>[2x]EEAEET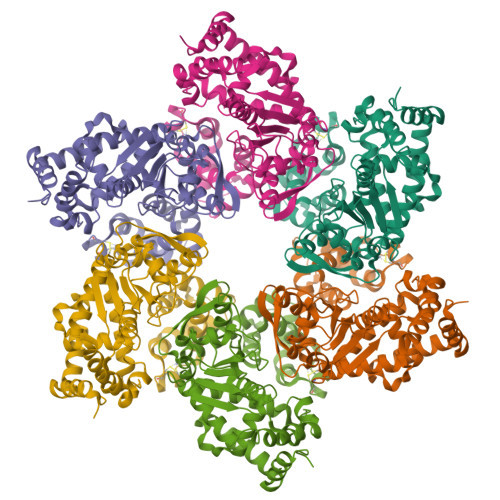KQVSWKLVTEYAMETKCDDVLLLLGMYLEFQYSFEMCLKCIKKEQPSHYKYHEKHYANAAIFADSKNQKTICQQAVDTVLAKKRVDSLQLTREQMLTNRFNDLLDRMDIMFGSTGSADIEEWMAGVAWLHCLLPKMDSVVYDFLKCMVYNIPKKRYWLFKGPIDSGKTTLAAALLELCGGKALNVNLPLDRLNFELGVAIDQFLVVFEDVKGTGGESRDLPSGQGINNLDNLRDYLDGSVKVNLEKKHLNKRTQIFPPGIVTMNEYSVPKTLQARFVKQIDFRPKDYLKHCLERSEFLLEKRIIQSGIALLLMLIWYRPVAEFAQSIQSRIVEWKERLDKEFSLSVYQKMKFNVAMGIGVLD7-AMINO-1-METHYL-3-(2-METHYL-5-{[3-(TRIFLUOROMETHYL)BENZOYL]AMINO}PHENYL)-2-OXO-2,3-DIHYDROPYRIMIDO[4,5-D]PYRIMIDIN-1-IUM | C22 H18 F3 N6 O2 | 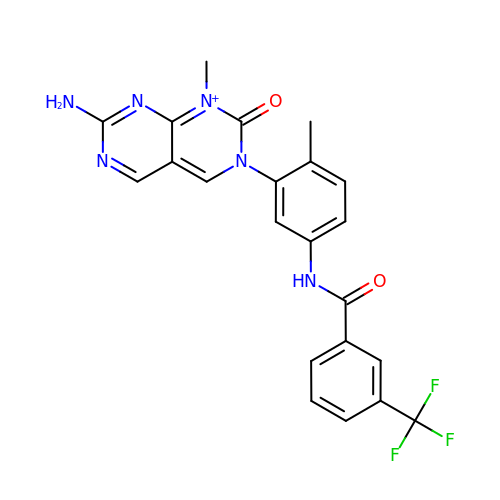SQOIIWIQKKMCCG-UHFFFAOYSA-O>[2x]MGSSYHHHHHHSSGENLYFQHMKHGRVFIIKSYSEDDIHRSIKYNIWCSTEHGNKRLDAAYRSMNGKGPVYLLFSVNGSGHFCGVAE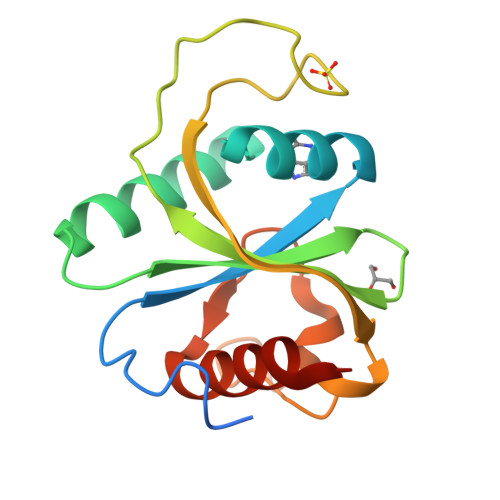MKSAVDYNTCAGVWSQDKWKGRFDVRWIFVKDVPNSQLRHIRLENNENKPVTNSRDTQEVPLEKAKQVLKIIASYKHTTS> MGSSHHHHHHSSGLVPRGGSHMSAASSIFDFEVL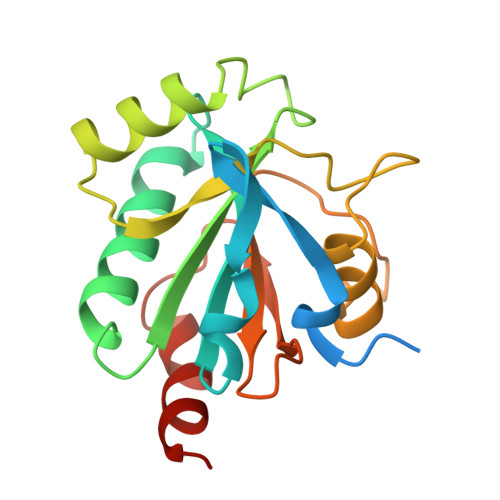DADHKPYNLVQHKGSPLLIYNVASKCGYTKGGYETATTLYNKYKSQGFTVLAFPCNQFGGQEPGNEEEIKEFVCTKFKAEFPIMAKINVNGENAHPLYEYMKKTKPGILKTKAIKWNFTSFLIDRDGVPVERFSPGASVKDIEKKLIPLLESTQSA> ESLYQSKYEELQITAGRHGDSVRNSKIEISELNRVIQRLRSEIDNVKKQISNLQQSISDAEQRGENALKDAKNKLNDLEDALQQA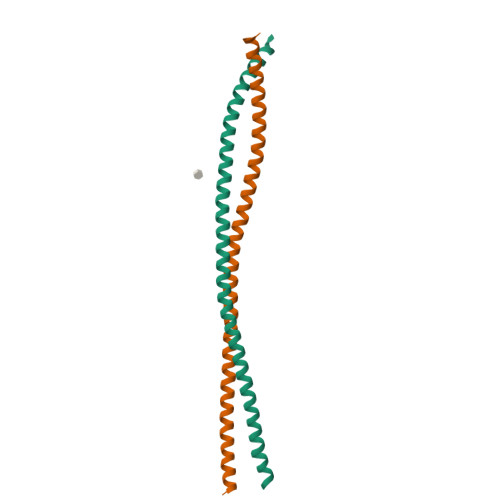KEDLARLLRDYQELMNTKLALDLEIATYRTLLEGE;> GSEAWFNEKSKELTTEIDNNIEQISSYKSEITELRRNVQALEIELQSQLALKQSLEASLAETEGRYAVQLSQIQAQISALEEQLQQIRAETECQNTEYQQLLDIKIRLENEIQTYRSLLEGE> GSMDYDFKVKLSSERERVEDLFEYEGCKVGRGTYGHVYKAKRKDGKDDKDYALKQIEGTGISMSACREIALLRELKHPNVISLQKVFLSHADRKVWLLFDYAEHDLWHIIKFHRASKANKKPVQLPRGMVKSLLYQILDGIHYLHANWVLHRDLKPANILVMGEGPERGRVKIADMGFARLFNSPLKPLADLDPVVVTFWYRAPELLLGARHYTKAIDIWAIGCIFAELLTSEPIFHCRQEDIKTSNPYHHDQLDRIFNVMGFPADKDWEDIKKMPEHSTLMKDFRRNTYTNCSLIKYMEKHKVKPDSKAFHLLQKLLTMDPIKRITSEQAMQDPYFLEDPLPTSDVFAGCQIPYPKREFLTEEEPDDKGDKK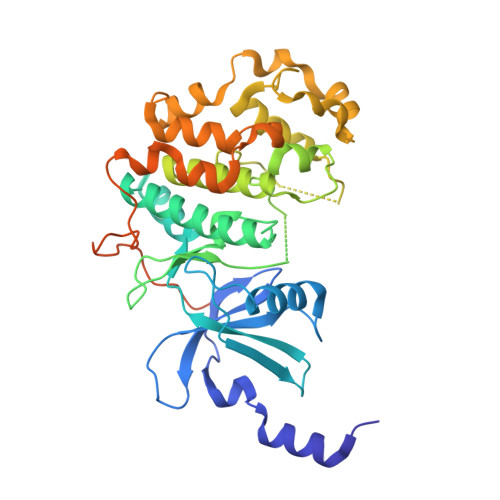NQQQQQGNNHTNGTGHPGNQDSSHTQGPPLKK> MPPQLHNGLDFSAKVIQGSLDSLPQEVRKFVEGNAQLCQPEYIHICDGSEEEYGRLLAHMQEEGVIRKLKKYDNCWLALTDPRDVARIQSKTVIITQEQRDTVPIPKSGQSQLGRWMSEEDFEKAFNARFPGCMKGRTMYVIPFSMGPLGSPLAKIGIELTDSPYVVASMRIMTRMGTSVLEALGDGEFIKCLHSVGCPLPLKKPLVNNWACNPELTLIAHLPDRREIISFGSGYGGNSLLGKKCFALRIASRLAKEEGWLAEHMLILGITNPEGKKKYLAAAFPSACGKTNLAMMNPTLPGWKVECVGDDIAWMKFDAQGNLRAINPENGFFGVAPGTSVKTNPNAIKTIQKNTIFTNVAETSDGGVYWEGIDEPLA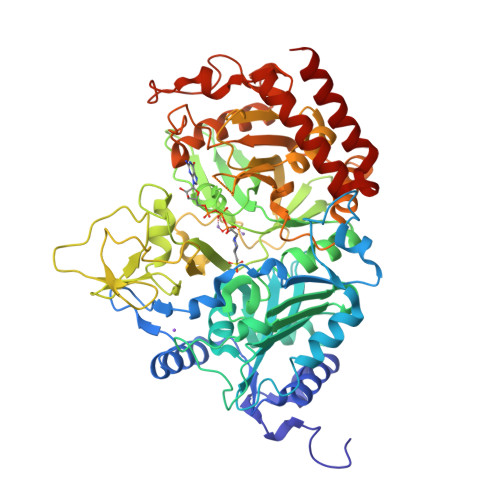PGVTITSWKNKEWRPQDEEPCAHPNSRFCTPASQCPIIDPAWESPEGVPIEGIIFGGRRPAGVPLVYEALSWQHGVFVGAAMRSEATAAAEHKGKVIMHDPFAMRPFFGYNFGKYLAHWLSMAHRPAAKLPKIFHVNWFRKDKNGKFLWPGFGENSRVLEWMFGRIEGEDSAKLTPIGYVPKEDALNLKGLGDVNVEELFGISKEFWEKEVEEIDKYLEDQVNADLPYEIERELRALKQRISQM>MKFGNFLLTYQPPELSQTEVMKRLVNLGKASEGCGFDTVWLLEHHFTEFGLLGNPYVAAAHLLGATETLNVGTAAIVLPTAHPVRQAEDVNLLDQMSKGRFRFGICRGLYDKDFRVFGTDMDNSRALMDCWYDLMKEGFNEGYIAADNEHIKFPKIQLNPSAYTQGGAPVYVVAESASTTEWAAERGLPMILSWIINTHEKKAQLDLYNEVATEHGYDVTKIDHCLSYITSVDHDSNRAKDICRNFLGHWYDSYVNATKIFDDSDQTKGYDFNKGQWRDFVLKGHKDTNRRIDYSYEINPVGTPEECIAIIQQDIDATGIDNICCGFEANGSEEEIIASMKLFQSDVMPYLKEKQ[2x];>MKFGLFFLNFMNSKRSSDQVIEEMLDTAHYVDQLKFDTLAVYENHFSNNGVVGAPLTVAGFLLGMTKNAKVASLNHVITTHHPVRVAEEACLLDQMSEGRFAFGFSDCEKSADMRFFNRPTDSQFQLFSECHKIINDAFTTGYCHPNNDFYSFPKISVNPHAFTEGGPAQFVNATSKEVVEWAAKLGLPLVFRWDDSNAQRKEYAGLYHEVAQAHGVDVSQVRHKLTLLVNQNVDGEAARAEARVYLEEFVRESYSNTDFEQKMGELLSENAIGTYEESTQAARVAIECCGAADLLMSFESMEDKAQQRAVIDVV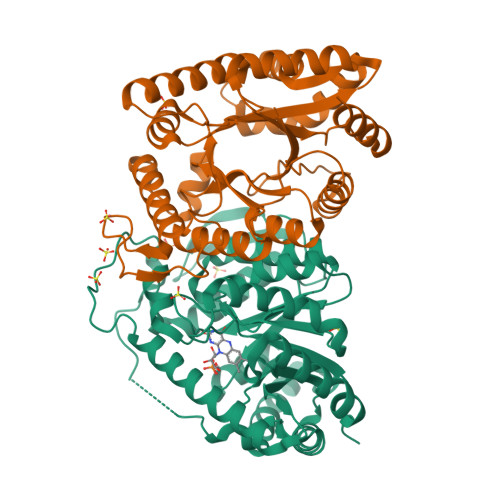NANIVKYHSLEHHHHHH[2x]3-ethyl-5-methyl-N-(5-methyl-1,2-oxazol-3-yl)-1,2-oxazole-4-carboxamide | C11 H13 N3 O3 | 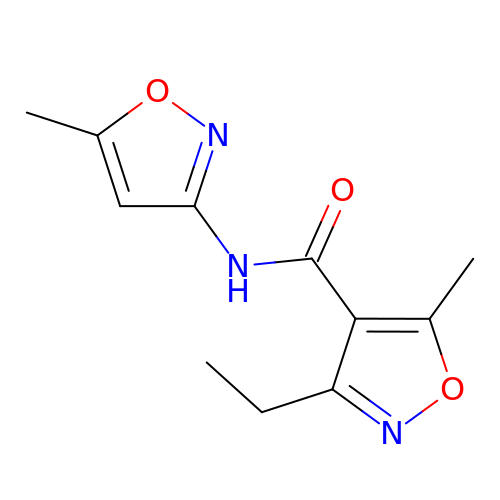OZMHRDLCZDDXRS-UHFFFAOYSA-N>[2x]MLDPNLLRNEPDAVAEKLARRGFKLDVDKLGALEERRKVLQVKTENLQAERNSRSKSIG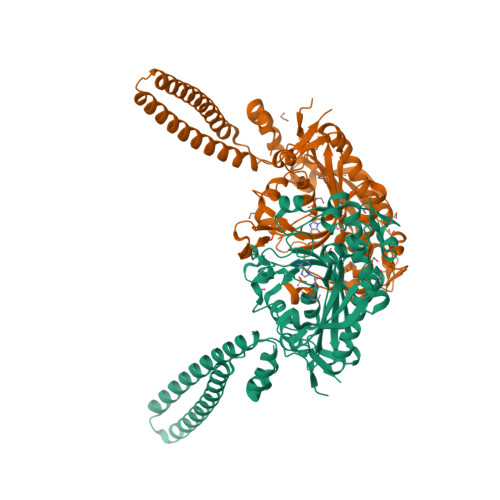QAKARGEDIEPLRLEVNKLGEELDAAKAELDALQAEIRDIALTIPNLPADEVPVGKDENDNVEVSRWGTPREFDFEVRDHVTLGEMHSGLDFAAAVKLTGSRFVVMKGQIARMHRALSQFMLDLHTEQHGYSENYVPYLVNQDTLYGTGQLPKFAGDLFHTRPLEEEADTSNYALIPTAEVPLTNLVRGEIIDEDDLPIKMTAHTPCFRSEAGSYGRDTRGLIRMHQFDKVEMVQIVRPEDSMAALEEMTGHAEKVLQLLGLPYRKIILCTGDMGFGACKTYDLEVWIPAQNTYREISSCSNVWDFQARRMQARCRSKSDKKTRLVHTLNGSGLAVGRTLVAVMENYQQADGRIEVPEVLRPYMNGLEYIGELALVPR> GSLRQEDFPPRIVEHPSDLIVSKGEPATLNCKAEGRPTPTIEWYKGGERVETDKDDPRSHRMLLPSGSLFFLRIVHGRKSRPDEGVYVCVARNYLGEAVSHDASLEVAILRDDFRQNPSDVMVAVGEPAVMECQPPRGHPEPTISWKKDGSPLDDKDERITIRGGKLMITYTRKSDAGKYVCVGTNMVGERE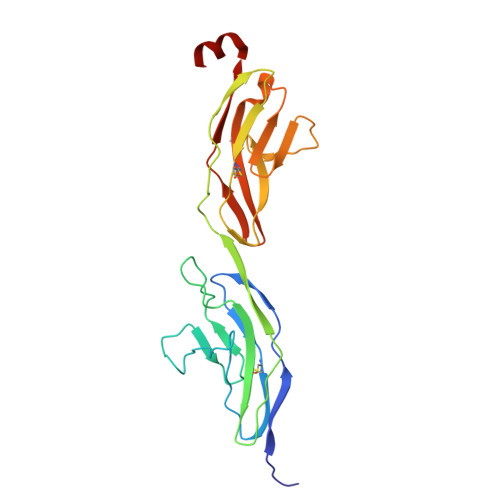SEVAELTVLERPSFVKAAAH> AMAAAEQQQFYLLLGNLLSPDNVVRKQAEETYENIPGQSKITFLLQAIRNTTAAEEARQMAAVLLRRLLSSAFDEVYPALPSDVQTAIKSELLMIIQMETQSSMRKKVCDIAAELARNLIDEDGNNQWPEGLKFLFDSVSSQNVGLREAALHIFWNFPGIFGNQQQHYLDVIKRMLVQCMQDQEHPSIRTLSARATAAFILANEHNVALFKHFADLLPGFLQAVNDSCYQNDDSVLKSLVEIADTVPKYLRPHLEATLQLSLKLCGDTSLNNMQRQLALEVIVTLSETAAAMLRKHTNIVAQTIPQMLAMMVDLEEDEDWANADELEDDDFD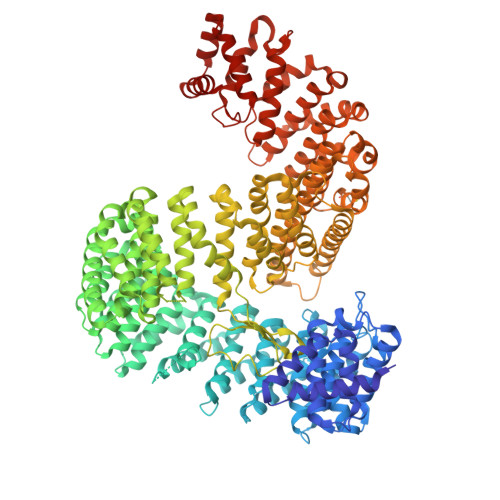SNAVAGESALDRMACGLGGKLVLPMIKEHIMQMLQNPDWKYRHAGLMALSAIGEGCHQQMEGILNEIVNFVLLFLQDPHPRVRYAACNAVGQMATDFAPGFQKKFHEKVIAALLQTMEDQGNQRVQAHAAAALINFTEDCPKSLLIPYLDNLVKHLHSIMVLKLQELIQKGTKLVLEQVVTSIASVADTAEEKFVPYYDLFMPSLKHIVENAVQKELRLLRGKTIECISLIGLAVGKEKFMQDASDVMQLLLKTQTDFNDMEDDDPQISYMISAWARMCKILGKEFQQYLPVVMGPLMKTASIKPEVALLDTQDMENMSDDDGWEFVNLGDQQSFGIKTAGLEEKSTACQMLVCYAKELKEGFVEYTEQVVKLMVPLLKFYFHDGVRVAAAESMPLLLECARVRGPEYLTQMWHFMCDALIKAIGTEPDSDVLSEIMHSFAKCIEVMGDGCLNNEHFEELGGILKAKLEEHFKNQELRQVKRQDEDYDEQVEESLQDEDDNDVYILTKVSDILHSIFSSYKEKVLPWFEQLLPLIVNLICPHRPWPDRQWGLCIFDDVIEHCSPASFKYAEYFLRPMLQYVCDNSPEVRQAAAYGLGVMAQYGGDNYRPFCTEALPLLVRVIQSADSKTKENVNATENCISAVGKIMKFKPDCVNVEEVLPHWLSWLPLHEDKEEAVQTFNYLCDLIESNHPIVLGPNNTNLPKIFSIIAEGEMHEAIKHEDPCAKRLANVVRQVQTSGGLWTECIAQLSPEQQAAIQELLNSA>[2x]GSGAAGTTTTSVTVHKLLATDGDMDKIANELETGNYAGNKVGVLPANAKEIAGVMFVWTNTNNEIIDENGQTLGVNIDPQTFKLSGAMPATAMKKLTEAEGAKFNTANLPAAKYKIYEIHSLSTYVGEDGATLTGSKAVPIEIELPLNDVVDAHVYPKNTEAKPKIDKDFKGKANPDTPRVDKDTPVNHQVGDVVEYEIVTKIPALANYATANWSDRMTEGLAFNKGTVKVTVDDVALEAGDYALTEVATGFDLKLTDAGLAKVNDQNAEKTVKITYSATLNDKAIVEVPESNDVTFNYGNNPDHGNTPKPNKPNENGDLTLTKTWVDATGAPIPAGAEATFDLVNAQTGKVVQTVTLTTDKNTVTVNGLDKNTEYKFVERSIKGYSADYQEITTAGEIAVKNWKDENPKPLDPTEPKVVTYGKKFVKVNDKDNRLAGAEFVIANADNAGQYLARKADKVSQEEKQLVVTTKDALDRAVAAYNALTAQQQTQQEKEKVDKAQAAYNAAVIAANNAFEWVADKDNENVVKLVSDAQGRFEITGLLAGTYYLEETKQPAGYALLTSRQKFEVTATSYSATGQGIEYTAGSGKDDATKVVNKKITI

One of the most prominent of these virulence factors is the bacterial pilus; a long, thin proteinaceous filament extending from the cell wall that aids bacterial colonisation in the nasopharynx through epithelial cell binding. In contrast, Gram-positive pili are formed from a single chain of covalently linked subunit proteins (pilins), usually comprising an adhesin at the distal tip, a major pilin that forms the polymer shaft and a minor pilin that mediates cell wall anchoring at the base. The 665-residue major pilin RrgB is solely responsible for the extended nature of the pilus, forming its polymeric shaft, which typically comprises 100–200 tandem RrgB molecules. In S. pneumoniae the genes required for pilus formation are located in the 12 kb rlrA islet and include three genes encoding proteins with the characteristic LPXTG motif. These correspond to the major pilin RrgB and two ancillary pilin proteins, the tip adhesin RrgA and the cell wall anchor protein RrgC.

Here we present the full-length crystal structure of the pneumococcal major pilin RrgB. RrgB was crystallized in space group P212121 and the structure was then solved at 2.8 Å resolution by molecular replacement, using the D2–D4 fragment as a search model. Two essentially identical RrgB molecules (root-mean square (rms) difference in Cα positions 0.61 Å) are present in the asymmetric unit. The structure of domains D2, D3 and D4 is unchanged from that seen for the previously-characterized D2–D4 fragment, with an rms difference of 0.86 Å for 442 Cα positions. A notable difference from the other major pilins so far characterized is that in RrgB domains D2 and D3 are packed side-by-side instead of end-on-end. D1 makes few contacts with D2, no contacts with D3, and in the crystal structure is offset from the plane formed from D2-D3-D4. The very small number of contacts between D1 and the rest of the structure suggests that in solution there is likely to be some flexibility in the orientation of D1 relative to D2–D4. The measured mass of RrgB of 64778.40 was ∼51 Da less than the theoretical value of 64829.34, indicating the presence of three isopeptide bonds. This was the same as previously observed for domains D2–D4, and is consistent with the formation of isopeptide bonds between Lys193-Asn318, Lys349-Asn428 and Lys453-Asn623, in domains D2, D3 and D4 respectively. We further show that absence of an internal isopeptide bond in the D1 domain arises because the β-strand carrying the Asn residue is displaced away from the position required for bond formation.Seneca virus A (SVA) is an emerging novel picornavirus that has recently been identified as the causative agent of many cases of porcine vesicular diseases in multiple countries. The full-length SVA genome is approximately 7.3 kb in length and contains a single open reading frame (ORF) encoding a single polyprotein that undergoes proteolytic processing and cleavage by the viral 3C protease (3Cpro) into four structural proteins (VP4-VP2-VP3-VP1) and eight non-structural proteins (L-2A-2B-2C-3A-3B-3C-3D). SVA 3Cpro is composed of two topologically equivalent antiparallel six-stranded β-barrel domains (A1-F1 and A2-F2). Three closely positioned residues (His48, Asp84 and Cys160) within the proteolytic active site of SVA 3Cpro comprise the canonical catalytic triad.

In the catalytically inactive C160A mutant structure, a phospholipid-like molecule could not be built due to lack of interpretable electron density data. In PV 3Cpro, the protease activity and RNA/lipid-binding are mutually regulated and the two sites are dynamically coupled. Similarly, we presumed that mutation of Cys160 may affect phospholipid-binding and partial phospholipids may be dynamically separated from the binding region; Therefore, the mutant could be used for phospholipid detection. As expected, the C160A mutant showed strong binding to cardiolipin (CL) as well as to phosphoinositol-4-phosphate (PI4P) and sulfatide, but displaying weak bindings to other categories of phospholipids, such as phosphatidic acid (PA), phosphatidylserine (PS) and phosphatidylethanolamine (PE). By quantitatively analyzing the intensities of the three positive spots, we demonstrated that the binding intensity to CL is 2-3-fold that of PI4P and sulfatide. Thus, CL is likely the dominant category of phospholipid that binds to SVA 3Cpro. In addition, the CL content in the C160A mutant was only ~40% of the wild-type, confirming that mutation of Cys160 affected lipid-binding and that the lipid could therefore not be modelled in C160A structure. The preferred binding of SVA 3Cpro to the CL may therefore explain the observation that a portion of C160A mutant can traffic to the mitochondria.

> QPNVDMGFEAAVAKKVVVPITFMVPNRPSGLTQSALLVTGRTFLINEHTWSNPSWTSFTIRGEVHTRDEPFQTVHFTHHGIPTDLMMVRLGPGNSFPNNLDKFGLDQMPARNSRVVGVSSSYGNFFFSGNFLGFVDSITSEQGTYARLFRYRVTTYKGWAGSALVCEAGGVRRIIGLHSAGAAGIGAGTYISKLGLIKALKHLGEPLATMQ>[2x]GAMGSMRCVVFNLREEEAPYVEKWKQSHPGVVVDTYEEPLTAKNKELLKGYEGLVVMQFLAMEDEVYDYMGACKLKVLSTRTAGFDMYNATLLKKHGIRLTNVPSYSPNAIGEYALAAALQLTRHAREIETFVRKRDFRWQKPI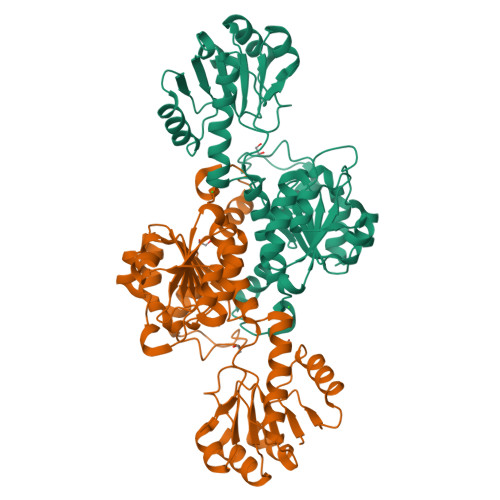LSKELRCSRVGILGTGRIGQAAARLFKGVGAQVVGFDPYPNDAAKEWLTYVSMDELLSTSDVISLHMPATKDSHHLINAKTIAQMKDGVYLVNTARGAVIDSQALLDSLDKGKIAGAALDAYEFEGPYIPKDNGNNPITDTVYARLVAHERIIYTPHIAFYTETAIENMVFNSLDACTTVLRGEPCAAEIKL>[2x]SNAMIEPGSKLVMVGDSITDCGRAHPVGEAPRGGLGNGYVALVDAHLQVLHPDWRIRVVNVGTSGNTVADVARRWEDDVMA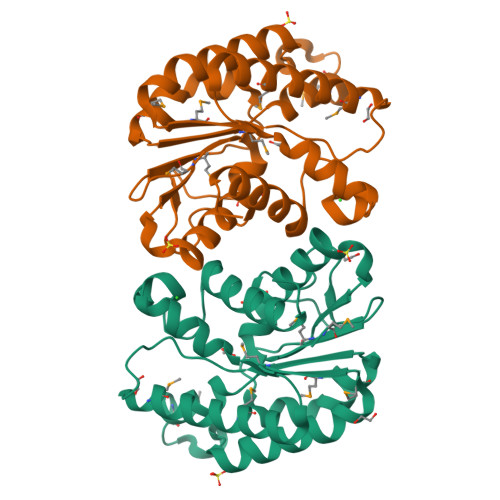LQPDYVSLMIGVNDVWRQFDMPLVVERHVGIDEYRDTLRHLVATTKPRVREMFLLSPFYLEPNRSDPMRKTVDAYIEAMRDVAASEHVPFVDVQAEFDRLLAHLNTWVLAPDRVHPYLNGHLVIARAFLTAVGVL>MAEAASCARKGTKYAEGTQPFTVLIEGNIGSGKTTYLNHFEKYKNDICLLTEPVEKWRNVNGVNLLELMYKDPKKWAMPFQSYVTLTMLQSHTAPTNKKLKIMERSIFSARYCFVENMRRNGSLEQGMYNTLEEWYKFIEESIHVQADLIIYLRTSPEVAYERIRQRARSEESCVPLKYLQELHELHEDWLIH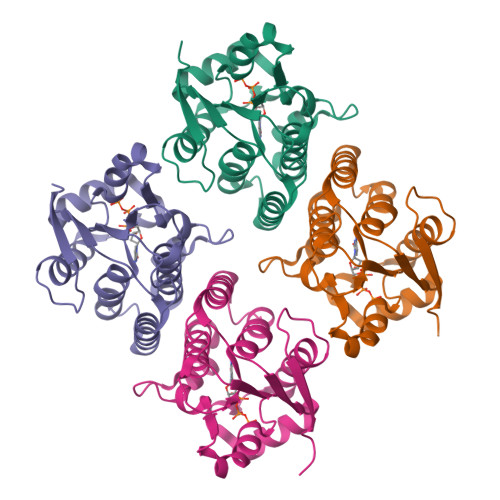QRRPQSCKVLVLDADLNLENIGTEYQRSESSIFDAIS[4x]>GHMSTLLINQ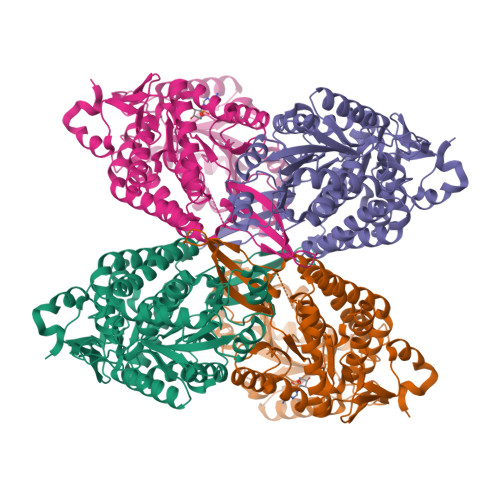PQYAWLKELGLREENEGVYNGSWGGRGEVITTYCPANNEPIARVRQASVADYEETVKKAREAWKIWADIPAPKRGEIVRQIGDALREKIQVLGSLVSLEMGKILVEGVGEVQEYVDICDYAVGLSRMIGGPILPSERSGHALIEQWNPVGLVGIITAFNFPVAVYGWNNAIAMICGNVCLWKGAPTTSLISVAVTKIIAKVLEDNKLPGAICSLTCGGADIGTAMAKDERVNLLSFTGSTQVGKQVGLMVQERFGRSLLELGGNNAIIAFEDADLSLVVPSALFAAVGTAGQRCTTARRLFIHESIHDEVVNRLKKAYAQIRVGNPWDPNVLYGPLHTKQAVSMFLGAVEEAKKEGGTVVYGGKVMDRPGNYVEPTIVTGLGHDASIAHTETFAPILYVFKFKNEEEVFAWNNEVKQGLSSSIFTKDLGRIFRWLGPKGSDCGIVNVNIPTSGAEIGGAFGGEKHTGGGRESGSDAWKQYMRRSTCTINYSKDLPLAQGIKFQ[2x]> MTYKLYIMTFQNAHFGSGTLDSSKLTFSADRIFSALVLEALKMGKLDAFLAEANQDKFTLTDAFPFQFGPFLPKPIGYPKHDQIDQSVDVKEVRRQAKLSKKLQFLALEN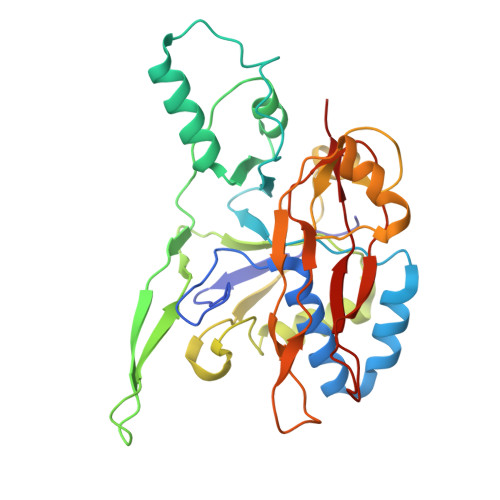VDDYLNGELFENEEHAVIDTVTKNQPHKDDNLYQVATTRFSNDTSLYVIANESDLLNELMSSLQYSGLGGKRSSGFGRFELDIQNIPLELSDRLTKNHSDKVMSLTTALPVDADLEEAMEDGHYLLTKSSGFAFSHATNENYRKQDLYKFASGSTFSKTFEGQIVDVRPLDFPHAVLNYAKPLFFKLEV>[3x]MPKIVILPHQDLCPDGAVLEANSGETILDAALRNG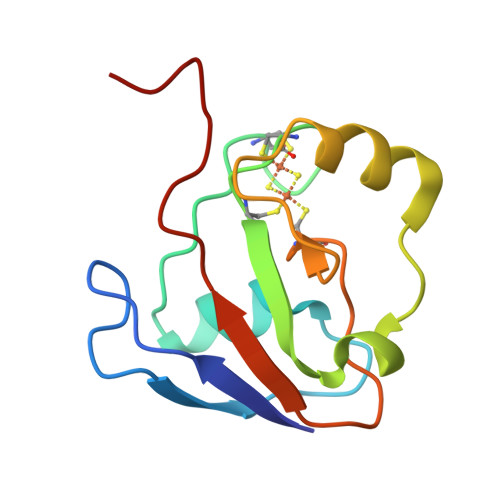IEIEHACEKSCACTTCHCIVREGFDSLPESSEQEDDMLDKAWGLEPESRLSCQARVTDEDLVVEIPRYTINHAREH>[4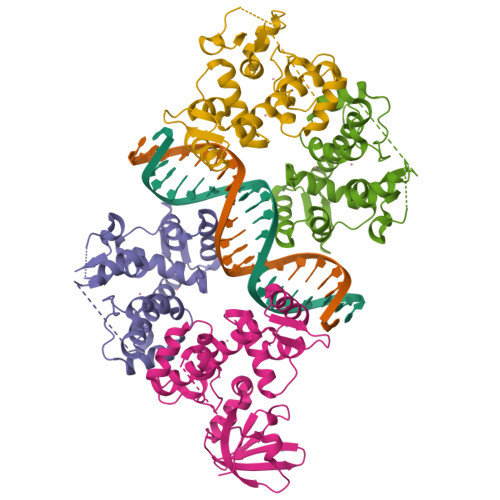x]KDLVDTTEMYLRTIYELEEEGVTPLRARIAERLEQSGPTVSQTVARMERDGLVVVASDRSLQMTPTGRTLATAVMRKHRLAERLLTDIIGLDINKVHDEACRWEHVMSDEVERRLVKVLKDVSRSPFGNPIPGLDELGVGNSDAAAPGTRVIDAATSMPRKVRIVQINEIFQVETDQFTQLLDADIRVGSEVEIVDRDGHITLSHNGKDVELLDDLAHTIRIEEL F17 and F18 fimbriae are wire-like structures expressed on the surface of enterotoxigenic and septicemic Escherichia coli (ETEC) strains that secrete toxins causing diarrhea in infantile livestock. F17, F18 and type-1 fimbriae are assembled by the chaperone/usher biogenesis pathway and comprise a few thousand copies of a major pilin (F17A, FedA and FimA respectively), several minor pilin proteins and a single two-domain adhesin (TDA) at the tip (F17G, FedF and FimH, respectively). The N-terminal domain of TDAs is a lectin domain, also called receptor-binding domain, because it mediates adherence of fimbriated bacteria to glycoconjugate receptors on host epithelial linings. Amino acid sequence and crystal structure analyses of the lectin domains of F17G, FedF and FimH elucidate a previously unacknowledged basis for strain-dependent glycan binding profiles of E. coli fimbrial adhesins, one that is driven by electrostatic interactions.

Surface Plasmon Resonance (SPR) interaction studies using a newly synthesized GlcNAcβ1-xGal series (x being 2, 3, 4 or 6) and F17G crystal structures in complex with these disaccharides provide insight in the structural basis of the variant-specific binding profiles. In each of these complexes, a terminal, non-reducing GlcNAc occupies the primary binding pocket in the same orientation as observed in the initial F17aG structure with GlcNAc. Near the non-reducing end of the disaccharide, Arg93 (purple) is bridging the GlcNAc residue and the sulfate ion S4, whereas variable residue Asn90 (cyan) of F17bG, substituted for Lys90 in F17aG, is bridging the O4 hydroxyl of the reducing galactose and the sulfate ion S4. The mutation in F17bG of Asn90 to Lys90 in F17aG could be at the basis of this observation, because a sulfate ion, S4, binds Asn90 in F17bG. The sulfate ion S4 is situated near the hydroxyl group at position 4 of galactose, where the disaccharide could be extended, towards the reducing end, into a larger oligosaccharide sequence. Variable residue Tyr114/Thr is located near the reducing end of the glycan and faces sulfate ion S1. The S2 sulfate ion binding site coincides exactly with a second GlcNAc binding site identified before in the crystal structure of F17cG, also called GafD. The F17G lectin domain sequences have been aligned elsewhere, however residue 110 of F17bG has been confirmed in the crystal structure to be a cysteine, not serine, that forms a disulfide bridge with Cys53. Interestingly, the addition of 10 mM GlcNAc-6-sulfate to crystals of F17bG instantly dissolves them.

> VVSFIGSTENDVGPSQGSYSSTHAMDNLPFVYNTGYNIGYQNANVWRIGGGFCVGLDGKVDLPVVGSLDGQSIYGLTEEVGLLIWMGDTNYSRGTAMSGNSWENVFSGWCVGNYLSTQGLSVHVRPVILKRNSSAQYSVQKTSIGSIRMRPYNGSSAGSVQTTVNFSLNPFTLNDT>MIDYTAAGFTLLQGAHLYAPEDRGICDVLVANGKIIAVASNIPSDIVPNCTVVDLSGQILCPGFIDQHVHLIGGGGEAGPTTRTPEVALSRLTEAGVTSVVGLLGTDSISRHPESLLAKTRALNEEGISAWMLTGAYHVPSRTITGSVEKDVAIIDRVIGVKCAISDHRSAAPDVYHLANMAAESRVGGLLGGKPGVTVF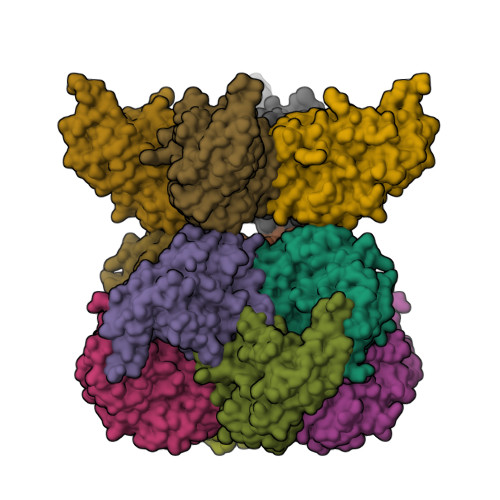HMGDSKKALQPIYDLLENCDVPISKLLPTHVNRNVPLFEQALEFARKGGTIDITSSIDEPVAPAEGIARAVQAGIPLARVTLSSDGNGSQPFFDDEGNLTHIGVAGFETLLETVQVLVKDYDFSISDALRPLTSSVAGFLNLTGKGEILPGNDADLLVMTPELRIEQVYARGKLMVKDGKACVKGTFETA[12x]> MLSPAGKISLQSFTGSSLVFFVICMFNHYYGITNLVVNTLIVFFYAVNVYFFLKFFYNEFAFAIAIRAAFLGLVLVLGLYIKLVAPPNIQIFGGYMSVMALFHYSEFLAIAIVQPKQVSTDSFVINHSPQYTIAAVSSWVEFFIETYFFPALKAIHWLSNIGLCVCILGEVLRKTAILTAGSNFNHLVQCEKSSDHVLVTHGVYAWFRHPSYVGWFYWSIGTQIIL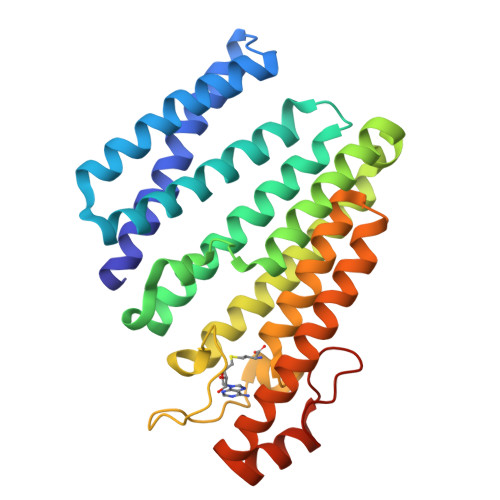INPLCIPAYTLASWMFFKERIYIEESMLLSFFGQQYCDYQQQVGTGIPFIEGYKIAAEGEEF>[10x]MENLNMDLLYMAAAVMMGLAAIGAAIGIGILGGKFLEGAARQPDLIPLLRTQFFIVMGLVDAIPMIAVGLGLYVMFAVA;>MNLNATILGQAIAFVLFVLFCMKYVWPPLMAAIEKRQKEIADGLASAERAHKDLDLAKASATDQLKKAKAEAQVIIEQANKRRSQILDEAKAEAEQERTKIVA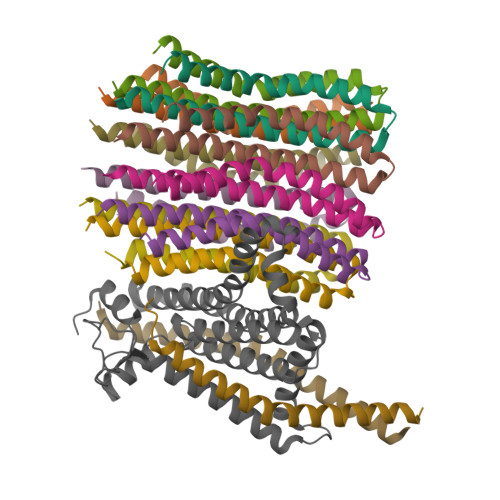QAQAEIEAERKRAREELRKQVAILAVAGAEKIIERSVDEAANSDIVDKLVAEL[2x];> MASENMTPQDYIGHHLNNLQLDLRTFSLVDPQNPPATFWTINIDSMFFSVVLGLLFLVLFRSVAKKATSGVPGKFQTAIELVIGFVNGSVKDMYHGKSKLIAPLALTIFVWVFLMNLMDLLPIDLLPYIAEHVLGLPALRVVPSADVNVTLSMALGVFILILFYSIKMKGIGGFTKELTLQPFNHWAFIPVNLILEGVSLLSKPVSLGLRLFGNMYAGELIFILIAGLLPWWSQWILNVPWAIFHILIITLQAFIFMVLTIVYLSMASEEH>[4x]GEFKG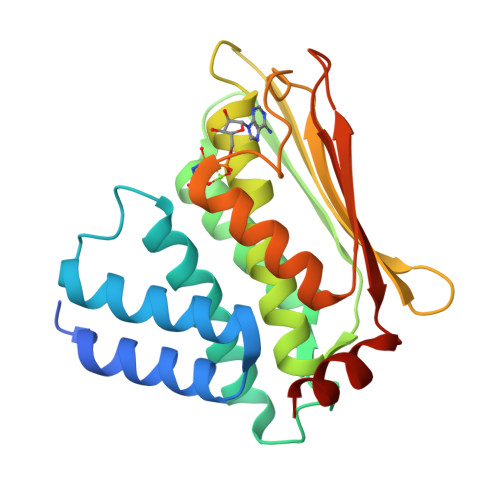LMGQSESPDRATELDRQLAEVQHRVKNHLAMIVSMIRIQSSQAGGVGSQFDSLSRRVEALQLLYQEMDIAGAAKATDKIIPLGAYLGRIASAINHIDGRGAIKVNVQADTVDVPVETAGRIGLLVSEVLTNALQHAFSDRASGVVQLRSSVMSGEQLRVTVEDDGRGIPEDCDWPNEGNLGSRIVRQLVQGLGAELNVTRGGTGTIVNIDIPLSQQKTLIADERTKD9-HYDROXYPROPYLADENINE, 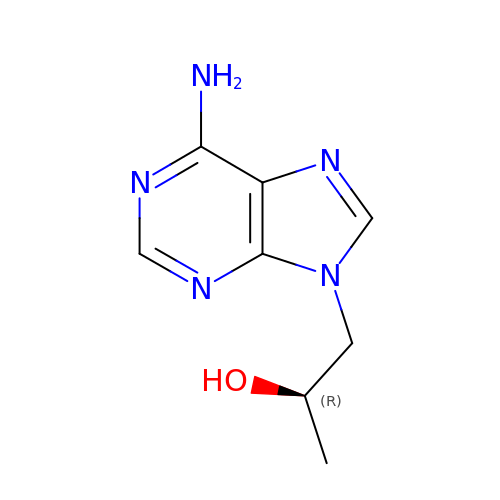R-ISOMER | C8 H11 N5 O | MJZYTEBKXLVLMY-RXMQYKEDSA-N>MSLKIAMIGLGDIAQKAYLPVLAQWPDIELVLCTRNPKVLGTLATRYRVSATCTDYRDVLQYGVDAVMIHAATDVHSTLAAFFLHLGIPTFVDKPLAASAQECENLYELAEKHHQPLYVGFNRRHIPLYNQHLSELAQQECGALRSLRWEKHRHALPGDIRTFVFDDFIHPLDSVNLSRQCNLDDLHLTYHMSEGLLARLDVQWQTGDTLLHASMNRQFGITTEHVTASYDNVAYLFDSFTQGKMWRDNQESRVALKDWTPMLASKGFDAMVQDWLQVAAAGKLPTHIIERNLASHQLAE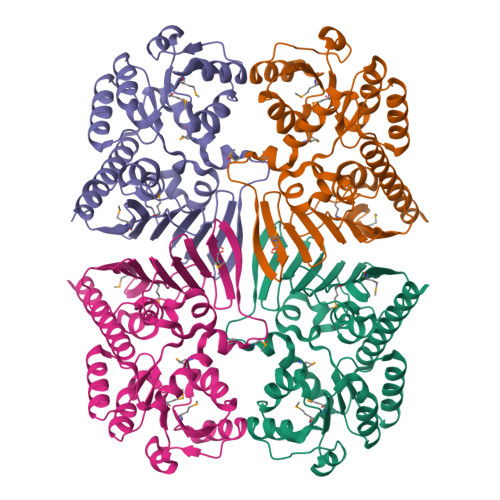AICQQITQQVTKGEGGSHHHHHH[4x]> PKLLNKFDKTIKAELDAAEKLRKRGKIEEAVNAFKELVRKYPQSPRARYGKAQCEDDLAEKRRSNEVLRGAIETYQEVASLPDVPADLLKLSLKRRSDRQQFLGHM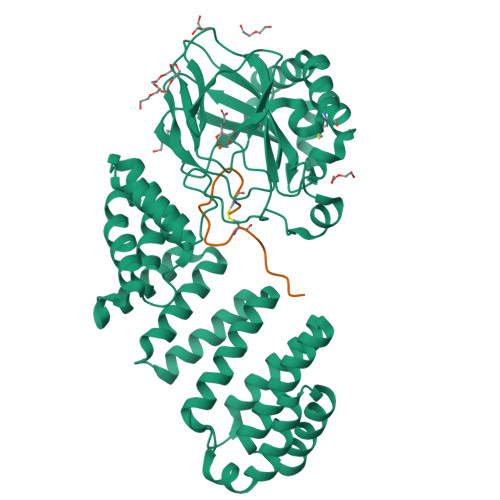RGSLLTLQRLVQLFPNDTSLKNDLGVGYLLIGDNDNAKKVYEEVLSVTPNDGFAKVHYGFILKAQNKIAESIPYLKEGIESGDPGTDDGRFYFHLGDAMQRVGNKEAYKWYELGHKRGHFASVWQRSLYNVNGLKAQPWWTPKETGYTELVKSLERNWKLIRDEGLAVMDKAKGLFLPEDENLREKGDWSQFTLWQQGRRNENACKGAPKTCTLLEKFPETTGCRRGQIKYSIMHPGTHVWPHTGPTNCRLRMHLGLVIPKEGCKIRCANETKTWEEGKVLIFDDSFEHEVWQDASSFRLIFIVDVWHPELTPQQRRSLPAI;> DGDQSETSPSQNQGKCKDGLGEYTCTSLEGFEGKNSELF N-{(1S)-1-[3-methoxy-4-(1,3-oxazol-5-yl)phenyl]ethyl}-N'-phenylurea 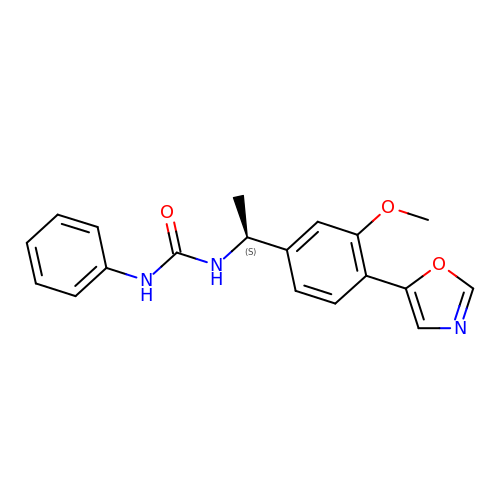| C19 H19 N3 O3 | UDNLNRJCNHAFEZ-ZDUSSCGKSA-N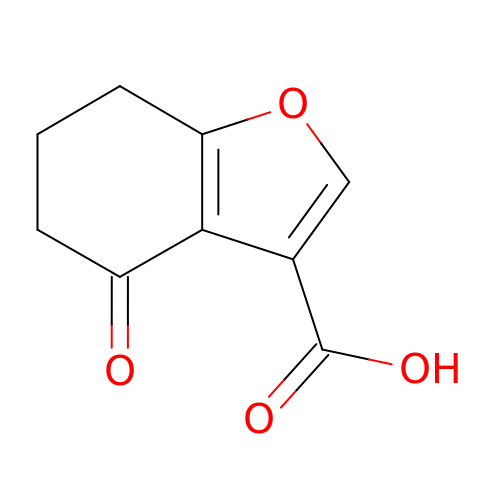4-oxo-4,5,6,7-tetrahydro-1-benzofuran-3-carboxylic acid | C9 H8 O4 | FABBWECRHZNMDQ-UHFFFAOYSA-N>MSNEIPKPVAPAPDILRCAYAELVVTDLAKSRNFYVDVLGLHVSYEDENQIYLRSFEEFIHHNLVLTKGPVAALKAMAFRVRTPEDVDKAEAYYQELGCRTERRKDGFVKGIGDALRVEDPLGFPYEFFFETTHVERLHMRYDLYSAGELVRLDHFNQVTPDVPRGRKYLEDLGFRVTEDIQDDEGTTYAAWMHRKGTVHDTALTGGNGPRLHHVAFSTHEKHNIIQICDKMGALRISDRIERGPGRHGVSNAFYLFILDPDNHRIEIYTQDYYTGD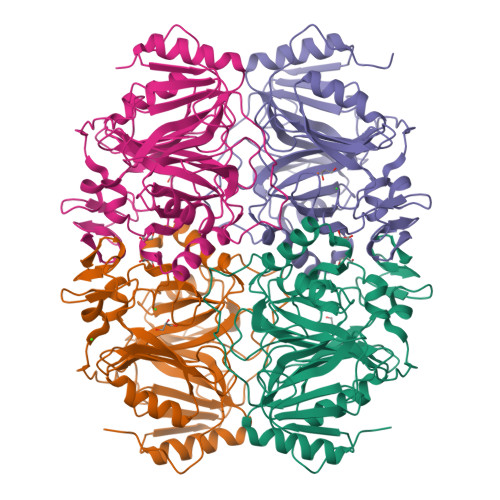PDNPTITWNVHDNQRRDWWGNPVVPSWYTEASKVLDLDGNVQEIIERTDDSELEVTIGADGFSFTRAGDEDGSYHGQASKGFKLGNQL[4x]>MRRVEKVIIVEGRSDKQKVAAVLNEPVVIVCTNGTISDARLEELADELEGYDVYLLADADEAGEKLRRQFRRMFPEAEHLYIDRAYREVAAAPIWHLAQV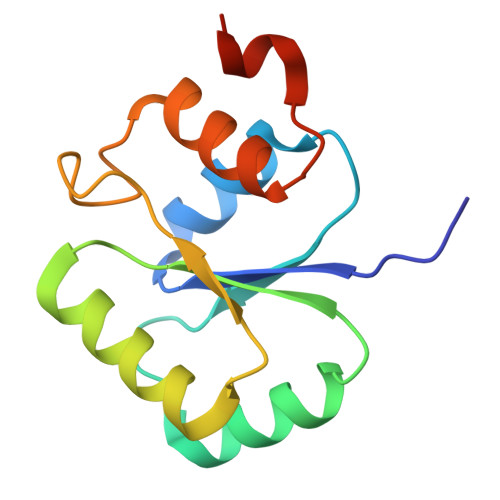LLRARFDVRIESLMRGRGE[3x]> MAFEDRDPTQFEERHLKFLQQLGKGNFGSVEMCRYDPLQDNTGEVVAVKKLQHSTEEHLRDFEREIEILKSLQHDNIVKYKGVCYSAGRR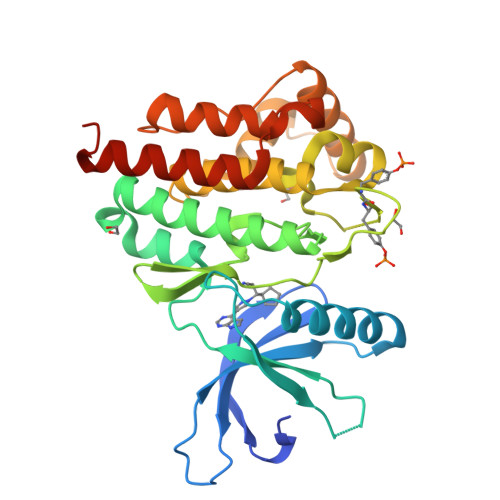NLKLIMEYLPYGSLRDYLQKHKERIDHIKLLQYTSQICKGMEYLGTKRYIHRDLATRNILVENENRVKIGDFGLTKVLPQDKEYYKVKEPGESPIFWYAPESLTESKFSVASDVWSFGVVLYELFTYIEKSKSPPAEFMRMIGNDKQGQMIVFHLIELLKNNGRLPRPDGCPDEIYMIMTECWNNNVNQRPSFRDLALRVDQIRDNMAGGSGSENLYFQ> MHHHHHHITSLYKKAGFENLYFQGKKIGVVLSGCGVYDGTEIHEAVLTLLAIARSGAQAVCFAPDKPQADVINHLTGEAMAETRNVLIEAARITRGDIRPLSQAQPEELDALIVPGGFGAAKNLSNFASQGSECRVDSDVVALAKAMHQSGKPLGFICIAPAMLPKIFDFPLRLTIGT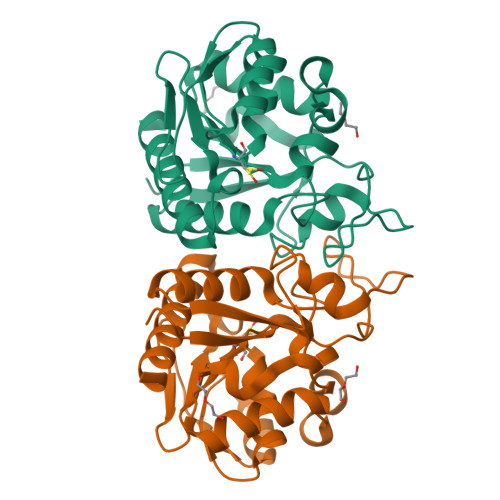DIDTAEVLEEMGAEHVPCPVDDIVVDEDNKVVTTPAYMLAQDIAQAASGIDKLVSRVLVLAE>MAEELVLERCDLELETNGRDHHTADLCREKLVVRRGQPFWLTLHFEGRNYQASVDSLTFSVVTGPAPSQEAGTKARFPLRDAVEEGDWTATVVDQQDCTLSLQLTTPANAPIGLYRLSLEASTGYQGSSFVLGHFILLFNAWCPADAVYLDSEEERQEYVLTQQGFIYQGSAKFIKNIPWNFGQFQDGILDICLILLDVNPKFLKNAGRDCSRRSSPVYVGRVGSGMVNCNDDQGVLLGRWDNNYGDGVSPMSWIGSVDILRRWKNHGCQRVKYGQCWVFAAVACTVLRCLGIPTRVVTNYNSAHDQNSNLLIEYFRNEFGEIQGDKSEMIWNFHCWVESWMTRPDLQPGYEGWQALDPTPQEKSEGTYCCGPVPVRAIKEGDLSTKYDAPFVFAEVNADVVDWIQQDDGSVHKSINRSLIVGLKISTKSVGRDEREDITHTYKYPEGSSEEREAFTRANHLNKLAEKEETGMAMRIRVGQSMNMGSDFDVFAHITNNTAEEYVCRLLLCAR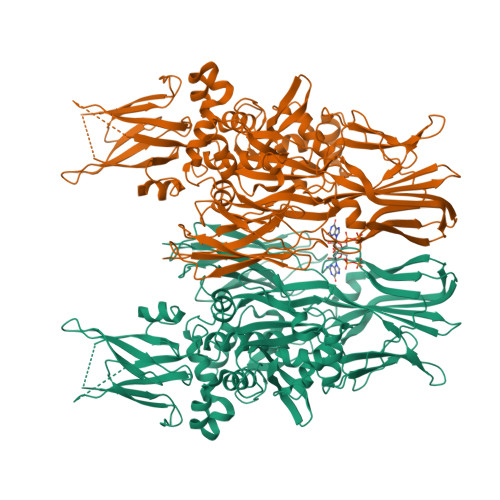TVSYNGILGPECGTKYLLNLTLEPFSEKSVPLCILYEKYRDCLTESNLIKVRALLVEPVINSYLLAERDLYLENPEIKIRILGEPKQKRKLVAEVSLQNPLPVALEGCTFTVEGAGLTEEQKTVEIPDPVEAGEEVKVRMDLVPLHMGLHKLVVNFESDKLKAVKGFRNVIIGPA[6x]> MLTLARQQQRQNIRWLLCLSVLMLLALLLSLCAGEQWISPGDWFTPRGELFVWQIRLPRTLAVLLVGAALAISGAVMQALFENPLAEPGLLGVSNGAGVGLIAAVLLGQGQLPNWALGLCAIAGALIITLILLRFARRHLSTSR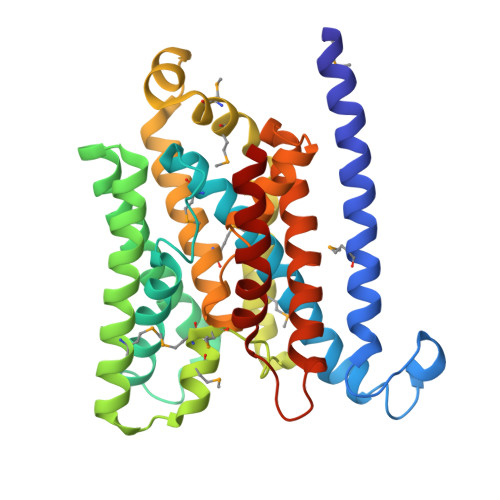LLLAGVALGIICSALMTWAIYFSTSVDLRQLMYWMMGGFGGVDWRQSWLMLALIPVLLWICCQSRPMNMLALGEISARQLGLPLWFWRNVLVAATGWMVGVSVALAGAIGFIGLVIPHILRLCGLTDHRVLLPGCALAGASALLLADIVARLALAAAELPIGVVTATLGAPVFIWLLLKAGR Thus, the BBSome is a key regulator of the composition of transmembrane proteins in the ciliary membrane, and is thought to be evolutionarily related to other transmembrane protein trafficking complexes including clathrin coats and the COPI and COPII coatomers. The recruitment of the BBSome to ciliary membranes (where it binds transmembrane protein substrates) is mediated by a highly specific interaction with ARL6 (also known as BBS3). Here, we use single-particle cryo-EM to determine structures of the native bovine BBSome complex with and without ARL6 at 3.5 Å and 3.1 Å resolution, respectively. The structures reveal the mechanism of ARL6-mediated activation and provide new insights into the pathogenesis of BBS-causing mutations and the evolutionary relationship between the BBSome and other transmembrane protein trafficking complexes.

In the absence of ARL6, the eight subunits of the BBSome are arranged in two lobes that we call the head and the body (referred to as the top and base lobes by Chou and colleagues [Chou et al., 2019]). The head is formed by an asymmetric heterodimer of BBS2 and BBS7, with the other six subunits forming the body. The head and body are connected by a helical neck formed from two abutting coiled coils, one from BBS2 and the other from BBS9. BBS1βprop occupies a special position in the BBSome, cradled loosely between BBS7 in the head and BBS4 in the body. Relative to the body, the head is more flexible and less well resolved, while BBS1βprop shows additional flexibility independent of the head movement. Within the body, BBS9 interacts with all other subunits of the BBSome. A crystal structure has shown that ARL6:GTP interacts with blades 1 and 7 of the BBS1βprop. However, this binding site is occluded in the BBSome structure, as blade 7 of BBS1 forms a continuous eight-stranded β-sheet with the corresponding blade of the adjacent BBS2βprop. BBS2βprop is unique among the BBSome β-propeller domains, as contains two Dx[D/N]xDG-like calcium-binding loops; the first in blade 4 and the second in blade 6. A calcium cation can be seen bound to both loops, coordinated by a network of acidic sidechains and the mainchain of the conserved glycine.

> MAETKSMFREVLPKQGQLYVEDITTMVLCKPKLLPLKSLTLEKLEKMQQAAQDTIHQQEMTEKEQKITH;> MAATSSSDSDGGKGESEANSKWLDSLSDSMANIHTFSACLALADFHGDGEYKLAMGDLGPDGRQPRLKVLKGHTLVSQKPLPDLPAAAVTFLMASHEPRTPALAIASGPCVYVYKNLKPYFKFSLPSLPTNPLEQDLWNQAKEDQIDPLTLKEMLEGIREKAEVPLSVQSLRFLPLELSEMEAFVNQHKSKSIRRQTVITTMTTLKKNLADEDAVSCLVLGTENKELLVLDPEAFTILAKMSLPSVPAFLEASGQFDVEFRLAAACRNGSIYILRRDSKRPKYCIELGAQPVGLVGVHKVLVVGSNQDSLHGFTYKGKRLWTVQMPAAILAMNLLEQHSRGLQAVMAALANEEVRIYHDKVLLNVIRTPEAVTSLCFGRYGREDNTLIMTTLGGGLIIKILKRTAVFAEGGGEAGPPPSQAIKLNVPRKTRLYVDQTLREREAGTAMHRTFQADLYLLRLRAARAYVQALESSLSPVSLTAREPLKLHAVVQGLGPTFKLTLHLQNTSTARPILGLVVCFLYNEVLYALPRAFFKVPLLVPGLNYPLETFVKSLSDKGISDIIKVLVLREGQSTPLLSAHINMPMSEGLAAD;> MLQPVFTLKLRHKISPRMVAVGRYDGTHPCLAAATQAGKVFIHNPHSRSQHLGAPRVLQSPLESDVSLLNINQTVSCLTAGVLNPELGYDALLVGTQTNLLAYDVYNNSDLFYREVADGASAIVLGTLGDITSPLAIIGGNCALQGFNHEGNDLFWTVTGDNVHSLALCDFDGDGKKELLVGSEDFDIRVFKEDEIVAEMSETEIITSLCPMYGSRFGYALSNGTVGVYDKTARYWRIKSKNQAMSIHAFDLNSDGVCELITGWSNGKVDARSDRTGEVIFKDNFSSAIAGVVEGDYRMEGCQQLICCSVDGEIRGYLPGTAEMRGNLMDISVEQDLIRELSQKKQNLLLELRNYEENAKAELSSPLNEADGHRGVIPANTKHHTALSVSLGSEAQAAHAELCISTSNDTIIRAVLIFAEGVFAGESHVVHPSVHHLSSSVRIPITPPKDIPVDLHLKTFVGYRSSTQFHVFELTRQLPRFSMYALTSPDPASEPLSYVNFIIAERAQRVVMWLNQNFLLPEDTNIQNAPFQVCFTSLRNGGQLYIKIKLSGEITVNTDDIDLAGDIIQSMASFFAIEDLQVEADFPVYFEELRKVLVKVDEYHSVHQKLSADMADNSNLIRSLLVQAEDARLMRDMKTMKNRYKELYDLNKDLLNGYKIRCNNHTELLGSLKAVNQAIQRAGHLRVGKPKNQVITACRDAIRSNNINMLFRIMRVGTASS;> MAEEKLSARTQLPVSAESQKPVLKKAPEFPILEKQNWLIHLYYIQKDYEACKAVIKEQLQETHGLCEYAIYVQALIFRLEGNIQESLRLFQMCAFLSPQCADNLKQVARSLFLLGKHKAAIEVYNEAAKLNQKDWEICHNLGVCYIYLKQFDKAQDQLHNALHLNRHDLTYIMLGKIFLLKGDLDKAIEIYKKAVEFSPENTELLTTLGLLYLQLGIYQKAFEHLGNTLTYDPTNYKAILAAGSMMQTHGDFDVALTKYKVVACAVIESPPLWNNIGMCFFGKKKYVAAISCLKRANYLAPLDWKILYNLGLVHLTMQQYASAFHFLSAAINFQPKMGELYMLLAVALTNLEDSENAKRAYEEAVRLDKCNPLVNLNYAVLLYNQGEKRDALAQYQEMEKKVNLLKYSSSLEFDPEMVEVAQKLGAALQVGEALVWTKPVKDPKSKHQTASTSKAAGFQQPLGSNQALGQAMSSAATCRKLSSGAGGTSQLTKPPSLPLEPEPTVEAQPTEASAQTREK;> MSVLDALWEDRDVRFDVSSQQMKTRPGEVLIDCLDSVEDTKGNNGDRGRLLVTNLRIVWHSLALPRVNLSIGYNCILNITTRTANSKLRGQTEALYVLTKCNSTRFEFIFTNLVPGSPRLYTSLIAVHRAYETSKMYRDFKLRSALIQNKQLRLLPQENVYNKINGVWNLSSDQGNLGTFFITNVRIVWHANMNDSFNVSIPYLQIRSVKIRDSKFGLALVIESSQQSGGYVLGFKIDPVEKLQESVKEINSLHKVYSANPIFGVDYEMEEKPQPLEALTVKQIQDDVEIDSDDHTDAFVAYFADGNKQQDREPVFSEELGLAIEKLKDGFTLQGLWEVMN;> MDLNLNRADYLQVGVTSQKTMKLLPASKHRATQKVVVGDHDGIVMCFGMKKGEAVTVFKTLPGQKIARLELGGALNTPQEKIFIAAGSEIRGFTKRGKQFLSFETNLTESIKAMHISGSDLFLSASYIYNHYCDCKDQHYYLSGDKINDVICLPVERLLREVPVLACQDRVLRVLQGSDVTYEIEVPGPPTVLALHNGNGGDSGEDLLFGTSDGKLGLIQITTSKPIHKWEIRNEKKRGGILCVDSFDIVGDGVKDLLVGRDDGMVEVYGFDNANEPVLRFDHTLSESVTSIQGGCVGKDGYDEIVVSTYSGWITGLTTEPVHKESGPGEELKFNQEMQNKISSLRSELEQLQYKVLQEREKYQQSSQSSKAKSAVPSFSVNDKFTLNKDDASYSLILEVQTAIDNVLIQSDVPIDLLDVDKNSAVVSFSSCDSESNDNFLLATYRCQANTTRLELKIRSIEGQYGTLQAYVTPRIQPKTCQVRQYHIKPLSLHQRTHFIDHDRPMNTLTLTGQFSFSELHSWVVFCMPEVPEKPPAGECVTFYFQNTFLDTQLESTYRKGEGVFKSDNISTISILKDVLSKEATKRKINLNISYEINEVSVKHTLKLIHPKLEYQLLLAKKVQLIDALKELQVHEGNTNFLIPEYRCILEEADHLQEEYKKQPAHLERLYGMITDLFIDKFKFKGTNVKTKVPLLLEILDSYDQNALIAFFDAA;> MEPLLLAWSYFRRRRFQLCADLCTQMLEKSPCDQAAWILKARALTEMVYVDEIDVDEEGIAEMILDENAIAQVPRPGTSLKLPGTNQTGGPSPAVRPVTQAGRPITGFLRPSTQSGRPGTIEQAIKTPRTAYTARPIASSSGRFVRLGTASMLTSPDGPFINLSRLNLAKYAQKPKLAKALFEYIFHHENDVKTALDLAALSTEHSQYKDWWWKVQIGKCYYRLGLYREAEKQFKSALKQQEMVDTFLYLAKVYISLDQPLTALNLFKQGLDKFPGEVTLLCGIARIYEEMNNISSATEYYKEVLKQDNTHVEAIACIGSNHFYTDQPEVALRFYRRLLQMGVYNCQLFNNLGLCCFYAQQYDMTLTSFERALSLAENEEEVADVWYNLGHVAVGTGDTNLAHQCFRLALVSNNQHAEAYNNLAVLEMRRGHVEQAKALLQTASSLAPHMYEPHFNFATISDKIGDLQRSYAAAKKSEAAFPDHVDTQHLIKQLEQHFAML;> MSLFKARDWWSTVLGDKEEFDQGCLCLADVDNTGNGQDKIIVGSFMGYLRIFNPHPVKTGDGAQAEDLLLEVHLRDPILQVEVGKFVSGTEMLHLAVLHSRKLCVYSVSGTLGNVEHGNQYQIKLMYEHNLQRTACNMTYGSFGGVKGRDLICIQSVDGMLMVFEQESYAFGRFLPGSLLPGPLAYSSRTDSFITVSSCHQVESYKYQVLAFATDADKRQETEQQKHGSGKRLVVDWTLNIGEQAIDICIVSFIQSASSVFVLGERNFFCLKDNGQIQFMKKLDYSPSCFLPYCSVSEGTINTLIGNHNNMLHIYQDVTLKWATQLPHVPVAVRVGCLHDLKGVIVTLSDDGHLQCSYLGTDPSLFQAPKVESRELNYDELDMELKELQKVIKNVNKSQDVWPLTEREDDLKVSAMVSPNFDSVSQATDVEVGADLVPSVTVKVTLKNRVALQKIKLSIYVQPPLVLTGDQFTFEFMAPEMTRTVGFSVYLKGSYSPPELEGNAVVSYSRPTERNPDGIPRVSQCKFRLPLKLVCLPGQPSKTASHKLTIDTNKSPVSLLSLFPGFAKQSEDDQVNVMGFRFLGGSQVTLLASKTSQRYRIQSEQFEDLWLITNELIIRLQEYFEKQGIKDFTCSFSGSVPLEEYFELIDHHFELRINGEKLEELLSERAVQFRAIQRRLLTRFKDKTPAPLQHLDTLLDGTYKQVIALADAVEENQDNLFQSFTRLKSATHLVILLIGLWQKLSADQIAILEAAFLPLQQDTQELGWEETVDAALSHLLKTCLSKSSKEQALNLNSQLGIPKDTSQLKKHITLFCDRLAKGGRLCLSTDAAAPQTMVMPGGCATIPESDLEGRSIDQDSSELFTNHKHLMVETPVPEVSPLQGVTE>[12x]MSIAVGMIETRGFPAVVEAADSMVKAARVTLVGYEKIGSGRVT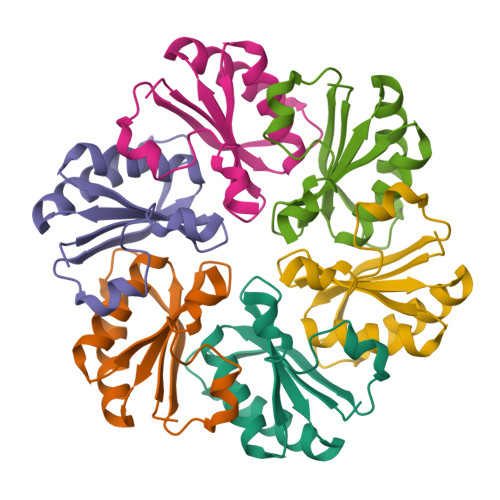VIVRGDVSGVQASVSAGIEAANRVNGGEVLSTHIIARPHENLEYVLPIRYTEEVEQFRTYGVPRGLEHHHHHH> DRSPGHHHHHHGGCPSQCSCSGTDVNCDGARFASVPAAIPITTQRLWLSNNQLTKLDPGVFDSLTQLTTLYLSNNQLTALPAGVFDKLTQLKELGLDQNQLKSIPDGAFARLPSLTHVWLHTNPWDCQCTDILYLSGWVAQHSSIVGEG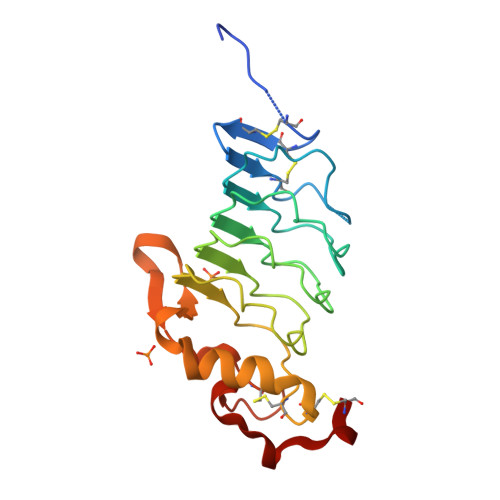WLRSWTVNPDNAKCSGTNTPVRAVTEASTSPSKCP ethyl 4-(2,3-dihydroindol-1-yl)-4-oxidanylidene-butanoate | C14 H17 N O3 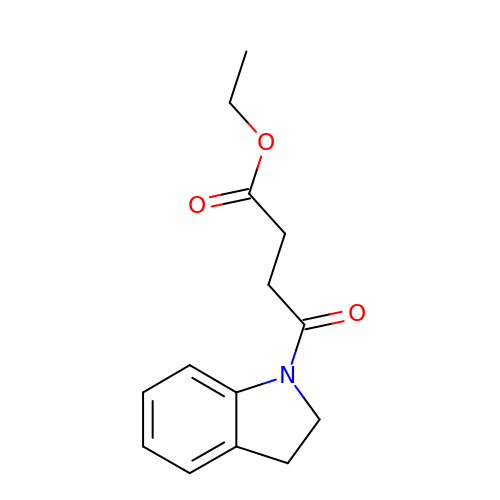| YTMPPLAKDQKOFM-UHFFFAOYSA-N5-[(5-{[4-{[4-(2-hydroxyethyl)piperazin-1-yl]methyl}-3-(trifluoromethyl)phenyl]carbamoyl}-2-methylphenyl)ethynyl]-1-methyl-1H-imidazole-2-carboxamide | C29 H31 F3 N6 O3 | 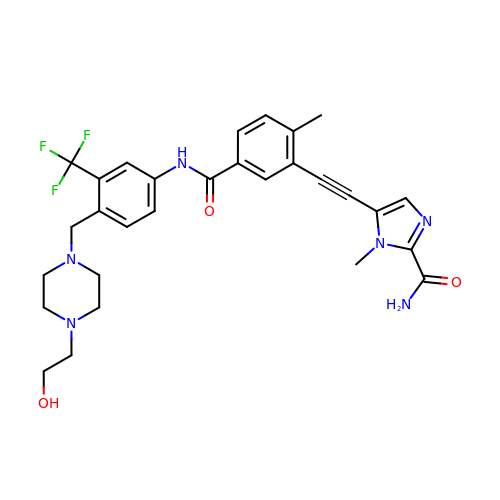GOLRXYBFRBKBAG-UHFFFAOYSA-N> MASMTGGQQMGRDEAGITGTWYNQLGSTFIVTAGADGALTGTYESAVGNAESRYVLTGRYDSAPATDGSGTALGWTVAWKNNYRNAHSATTWSGQYVGGAEARINTQWLLTA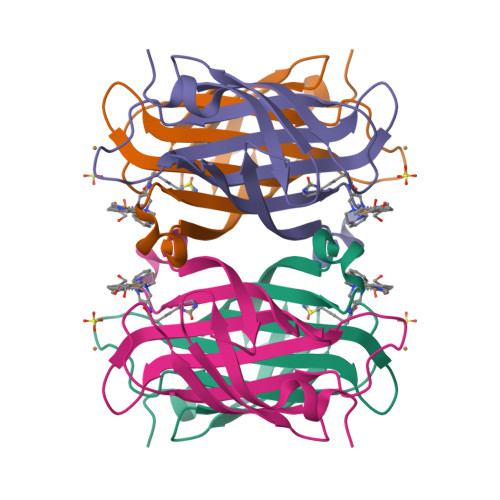GTTEANAWKSTLVGHDTFTKVKPSAASIDAAKKAGVNNGNPLDAVQQ>ACYCRIPACIAGERRAGTCIYQGRLWAACC[4x]

Defensins are a family of antimicrobial peptides of innate immunity broadly active against bacteria, viruses and toxins. They are small (2–5 kDa), stabilized structurally by three disulfide bonds, form oligomers, and are divided into α, β and θ structural classes. The canonical dimer interface of HNP1 is formed by the antiparallel extensions of the β2 strands stabilized by the reciprocal main-chain hydrogen bonds contributed by Thr18 and Ile20, and the hydrophobic packing of the side chains of Tyr16, Tyr21, Trp26, Phe28 and the Cys2–Cys30 and Cys4–Cys19 disulfides. Further analysis of probable quaternary structures by the Protein Interfaces, Surfaces and Assemblies (PISA) software indicates that the HNP1 dimer forms a tetramer or dimer of dimers in a crystal.

Analysis of HNP1 quaternary structures by PISA indicates that Tyr16 and Phe28 are essential for HNP1 dimerization contributing 16 and 11%, respectively, of the solvent-accessible surface buried by each monomer at the dimer interface. To further test the role of Tyr16 and Phe28 in mediating the HNP1 dimer, we prepared the double mutant Y16A/F28A-HNP1. Analysis of intermolecular contacts within the Y16A/F28A-HNP1 crystal indicates that mutant monomers assemble into compact dimers reassembling canonical dimers of wild-type HNP1. The replacement of the bulky side chains of Tyr16 and Phe28 by linear Ala side chains allows the dimer to pack more tightly and form an additional set of H-bonds on the opposite face of the dimer. The new set of four H-bonds pins the short β1 strand of one monomer to the equivalent strand of the other monomer to form a two-stranded antiparallel β-sheet. The significant increase in the average value of the molecular surface buried within inter-monomer interactions of Y16A/F28A-HNP1 as compared to the wild-type dimer is attributed to the presence of additional interactions mediated by the β1 strands. Introduction of mutations at the dimer interface have no effect on the ability of Y16A/F28A-HNP1 to form a stable tetramer, which closely resembles the wild type HNP1 tetramer. Unlike the F28A mutation alone, the Y16A/F28A double mutant and the quadruple mutant LF inhibition IC50 values increased 6-fold and 95-fold, respectively. In the virtual colony count assay, the double mutant Y16A/F28A-HNP1 had a vLD99.9 value against S. aureus 7-fold higher than HNP1, and Y16A/I20A/L25A/F28A-HNP1 failed to exhibit activity equivalent to the vLD90 level against S. aureus. The fact that the I20A/L25A double mutations were irrelevant, but the Y16A/F28A double mutations were quite relevant, for E. coli activity is insightful, because it demonstrates that the hydrophobicity of Tyr16 and Phe28 has repercussions beyond dimerization.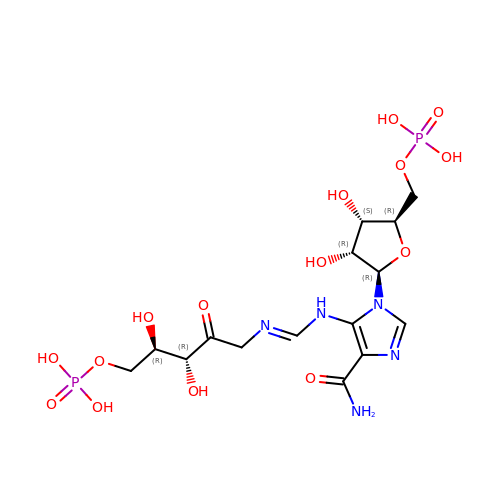[(2R,3S,4R,5R)-5-[4-AMINOCARBONYL-5-[[(Z)-[(3R,4R)-3,4-DIHYDROXY-2-OXO-5-PHOSPHONOOXY-PENTYL]IMINOMETHYL]AMINO]IMIDAZOL-1-YL]-3,4-DIHYDROXY-OXOLAN-2-YL]METHYL DIHYDROGEN PHOSPHATE | C15 H25 N5 O15 P2 | BLKFNHOCHNCLII-GHVQHMAVSA-N>MGSHHHHHHHHENLYFQSSLQKTAIETVNDMGLGWNLGNTFDCFGTWKEIKTPDDQITMWGNVVPTEEMVVTIKKYGFNTVRFPVTWMNFMDDSGNVNAEWMSRVKEVVDWIIKAGMYCILNVHHDGVSGNWLSQGASVKTKFVTLWTQIANEFKSYDDHLVLESMNEVEYKTGNDFDFTTLHTLTQAFVDTVRGTGGNNADRLLLISGMNTNLEQTCSSGYKMPTDKADKLAISIHYYLPPQFTVESDKNPWTWTDDQGVVHEITPMQTWGTESDYKEMVTNYETMKVTFADKGIPVILGEVGVLTEEQKDKDSIREFLYAQYSFS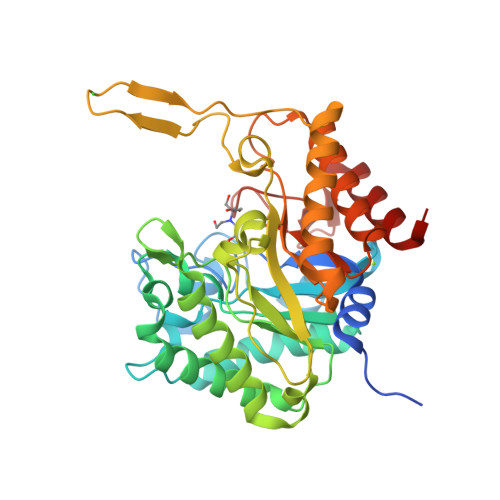AAYDGFMSVLWDTSKNTAGDMNFYNRETDKWYDEKIRDNFVNIAAGV[2x]> AIDEIKSRGYLLVGLSADFPPFEFVDENGNIVAFDVDLAKEIARRLGVELKIVDMTFDGLIPSLLTKKIDVIISGMTITEERKKVVAFSDPYFDAGQVIVVRKDSDFRPKTYEDLVGKTVAVQIGTTGDIEVSKYDGIKVVRFDKFTDAFLELKRGRADAVVLDSATARAFVAKNPDLVISSGVLSSEQYGIAVRKEDTDLLEFINSVLRELK

Among others, the arginine binding protein isolated from Thermotoga maritima (TmArgBP) contains one helix insertion motif, with Gly52 in the C0 position. The structural effects associated with the replacements of Gly residues adopting conformations forbidden to other residues were here evaluated using TmArgBP as model system. This protein is endowed with remarkable biophysical and structural properties, and presents a helix insertion motif located in the D1 domain. The helix insertion motif is locked by two consecutive C = O H-N H-bonds, made by residues Pro40-Phe53 and Phe41-Asp54. The Gly52 residue, which occupies the C0 position of the motif and presents a well-defined electron density in the crystal structures of TmArgBP variants, adopts a conformation that is strictly forbidden to non-Gly residues.

The Gly52 residue in C0 position was replaced either by Ala (TmArgBP20-233_G52A) or by Val (TmArgBP20-233_G52V). High resolution data, extending up to 1.64 Å resolution, were collected on TmArgBP20-233_G52A crystals. The TmArgBP20-233_G52A crystals contain one molecule in the asymmetric unit and, as expected, the protein presents an arginine molecule in the active site. Indeed, the root mean square deviation (RMSD) value computed on the Cα atoms between TmArgBP20-233_G52A and TmArgBP20-233 is as low as 0.29 Å, although the crystals used to solve these structures were not isomorphous. Determination of Ala52 main chain dihedral angle values (φ = 117.3°, ψ = −170.9°) indicates that Ala52 assumes a conformation closely similar to that of Gly52 in TmArgBP structures. This conformation falls in the ε region of the Ramachandran plot, and is considered to be strictly forbidden to non-Gly residues. Moreover, as in the parent protein, the carbonyl-oxygen of Ala52 forms an H-bond with the nitrogen of Asp56. In TmArgBP20-233_G52A the distances Ala52Cβ-Val51O and Ala52Cβ-Phe53N are 2.8 Å and 2.9 Å, respectively. Since it has been shown that backbone geometry may show a significant level of variability, the local valence bond geometry and deviations from planarity of the peptide bond have been compared with values detected in well refined protein structures. This analysis unravels the occurrence of significant deviations from average values for both peptide planarity and bond angles. Altogether these findings demonstrate that the significant destabilization induced by the Gly52Ala mutation is caused by apparently minimal structural perturbations.>[2x]MDTFVLDTSVFTNPDVYHQFEEDQLGAIENFISLASHTNANFFMPTSVYYEFTKMVSLGDLAPKFELV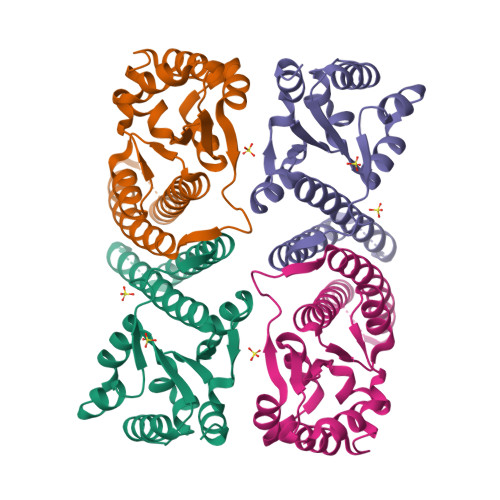VRIRSPRKWGLMVPAEFLYEFIEEVRYRINKGLRIAEEHTKEAGKLAEEEVGRVVNRLREKYREALRAGIIDSKEDVDVLLLSYELDAILVSGDEGLRKWADRVGIKLIDPKNLRYIMENLTKVGR> GSAESAISDISGSYVVPGTALQPLYQALDLPAEIVARAGRLTATVKVSQVDGRIDCETLLGNKTFRTSFVDGAVLETNGPERHNLSFDASQSTMAAGPFSLTYAASAAGLEVRYVAAGLDHRAVFAPGVSPRSAPG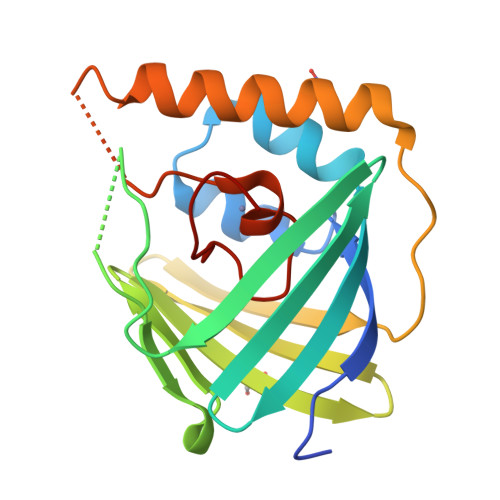EVTAFCSALYRFNREAQRLSLTGNFWFHPEGLLGPFAPFSPGHVWESA PIMELOYL-AMP | C17 H24 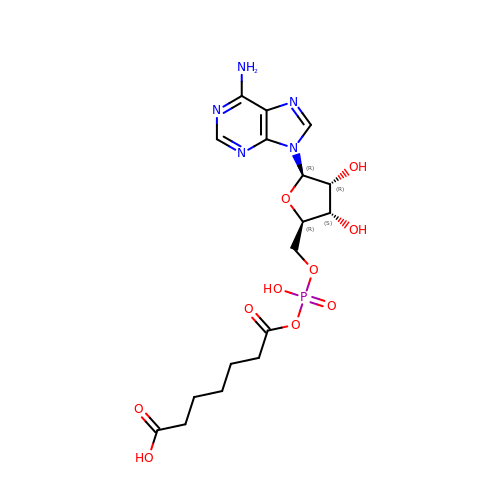N5 O10 P | CPQFOEZUJPOPAM-KRQFVHPKSA-N> MNALHRIGAGTLLAVLLAFGLTGCGEKEEVQQSLEPVAFHDSDE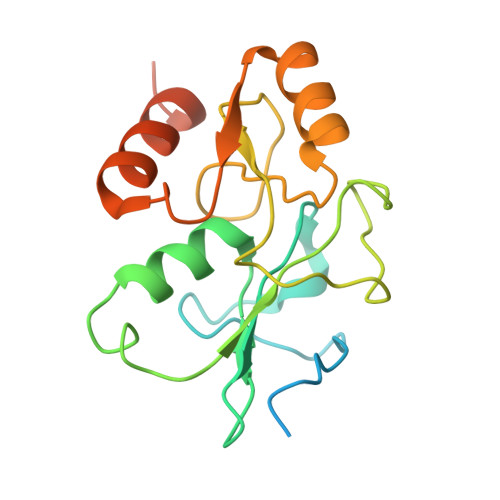CHVCGMIITDFPGPKGQAVEKRGVKKFCSTAEMLGWWLQPENRLLDAKLYVHDMGRSVWEKPDDGHLIDATSAYYVVGTSLKGAMGASLASFAEEQDAKALAGMHGGRVLRFEEIDQALLQEAASMQHGGMHDHAPNGAHNAHAGH> MMFGKKKNNGGSSTARYSAGNKYNTLSNNYALSAQQLLNASKIDDIDSMMGFERYVPPQYNGRFDAKDIDQIPGRVGWLTNMHATLVSQETLSSGSNGGGNSNDGERVTTNQGISGVDFYFLDEEGGSFKSTVVYDPYFFIACNDESRVNDVEELVKKYLESCLKSLQIIRKEDLTMDNHLLGLQKTLIKLSFVNSNQLFEARKLLRPILQDNANNNVQRNIYNVAANGSEKVDAKHLIEDIREYDVPYHVRVSIDKDIRVGKWYKVTQQGFIEDTRKIAFADPVVMAFAIATTKPPLKFPDSAVDQIMMISYMIDGEGFLITNREIISEDIEDFEYTPKPEYPGFFTIFNENDEVALLQRFFEHIRDVRPTVISTFNGDFFDWPFIHNRSKIHGLDMFDEIGFAPDAEGEYKSSYCSHMDCFRWVKRDSYLPQGSQGLKAVTQSKLGYNPIELDPELMTPYAFEKPQHLSEY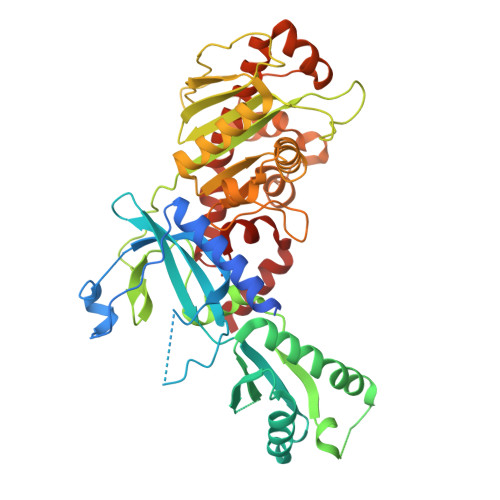SVSDAVATYYLYMKYVHPFIFSLCTIIPLNPDETLRKGTGTLCEMLLMVQA Nitrile hydratase (NHase, EC 4.2.1.84), comprising α- and β-subunits, is a metalloenzyme that catalyzes nitriles into amides. The NHase active site contains either a non-heme iron or non-corrin cobalt, buried in a deep internal pocket, similar to most enzymes in nature. Hence nitrile substrates should pass through a tunnel to access the active site, and rational tunnel engineering might be a plausible choice for NHase substrate scope modification. We rationally refined the tunnel entrance region of NHase from Pseudonocardia thermophila JCM 3095 (PtNHase), based on substrate access tunnel calculations.

Two successful mutants, PtNHase-βM46R and PtNHase-βA129R, which exhibited high catalytic activity toward bulky substrates were obtained. To understand the mechanism underlying the expanded substrate scope with bulky amino acid substituents, the crystal structures of PtNHase-βM46R and PtNHase-βA129R were obtained and analyzed. Both structures had clear electron density at the mutated sites. The βArg46 and βArg129 residues were located at the “upper entrance loop” and “lower entrance loop” of the substrate access tunnel, respectively. No interactions were observed between β129A and its surrounding residues in the WT, and the side chain of β129A was also buried and oriented towards the interior of the protein. In the case of PtNHase-βA129R, the side chain of βArg129 formed a salt-bridge with βAsp49, which maintained the side chain of the Arg129 outward offset from the substrate access tunnel. In addition, entrance shape and size analysis indicated that the entrance of the PtNHase-βA129R was expanded compared to that of its parent enzyme. Introducing β46R and β129R mutations into PtNHase resulted in an 8.2-fold and 4.2-fold increase in activity toward pentanenitrile, and a 6.2-fold and 8.3-fold increase in activity toward cinnamonitrile, respectively. However, the PtNHase-βA129R mutant lost more than half of its initial activity, suggesting that it is a stability–activity trade-off mutant. The maximum entrance sizes of WT, PtNHase-βM46R, and PtNHase-βA129R were estimated to be 39 Å2, 47 Å2, and 46 Å2, respectively.

> MTENILRKSDEEIQKEITARVKALESMLIEQGILTTSMIDRMAEIYENEVGPHLGAKVVVKAWTDPEFKKRLLADGTEACKELGIGGLQGEDMMWVENTDEVHHVVVCTLCSCYPWPVLGLPPNWFKEPQYRSRVVREPRQLLKEEFGFEVPPSKEIKVWDSSSEMRFVVLPQRPAGTDGWSEEELATLVTRESMIGVEPAKAVA;> MNGVYDVGGTDGLGPINRPADEPVFRAEWEKVAFAMFPATFRAGFMGLDEFRFGIEQMNPAEYLESPYYWHWIRTYIHHGVRTGKIDLEELERRTQYYRENPDAPLPEHEQKPELIEFVNQAVYGGLPRSREVDRPPKFKEGDVVRFSTASPKGHARRARYVRGKTGTVVKHHGAYIYPDTAGNGLGECPEHLYTVRFTAQELWGPEGDPNSSVYYDCWEPYIELVDTKAAAA>MTPPESPTASHTPGATPPRDFPIQRGCPFAAPAEYAALRTDDPVARVTLPTRREAWVVTRYDDVRELLSDPRVSADIRRPGFPALGEGEQEAGARFRPFIRTDAPEHTRYRRMLLPAFTVRRVRAMRPAVQARVDEILDGMLAAGGPVDLVSAYANAVSTSVICELLGIPRHDLEFFRDVTRISGSRNSTAEQVSEALGGLFGLLGGLVAERREEPRDDLISKLVTDHLVPGNVTTEQLLSTLGITINAGRETTTSMIALSTLLLLDRPELPAELRKDPDLMPAAVDELLRVLSVADSIPLRVAAEDIELSGRTVPADDGVIALLAGANHDPEQFDDPERVDFHRTDNHHVAFGYGVHQCVGQHLARLELEVALETLLRRVPTLRLAGERDQVVVKHDSATFGL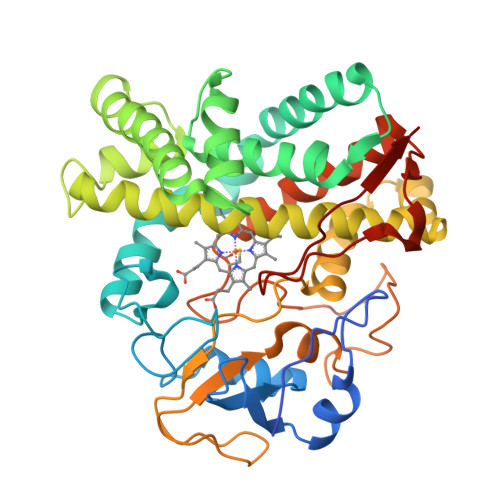EELMVTWHHHHHH[2x]> TSENPKIGPISEVASGVKTTANGIERIPVIGEIAKPVTTAVK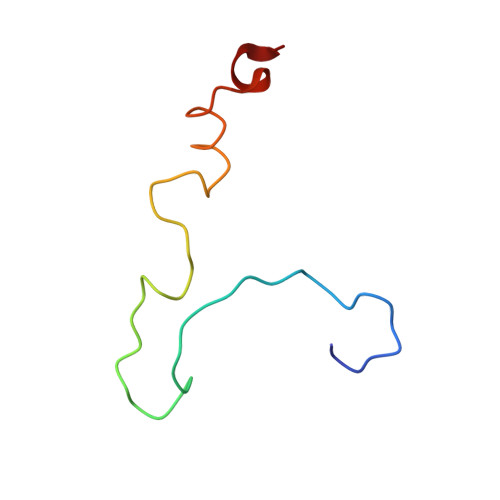WFADVVGTVAAIFGW>[2x]QTSVSPSKVIL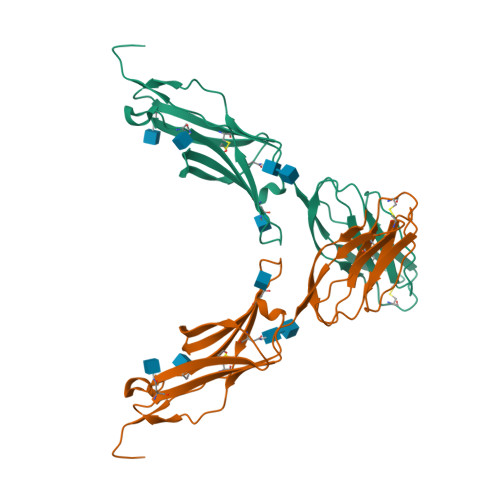PRGGSVLVTCSTSCDQPKLLGIETPLPKKELLLPGNNRKVYELSNVQEDSQPMCYSNCPDGQSTAKTFLTVYWTPERVELAPLPSWQPVGKNLTLRCQVEGGAPRANLTVVLLRGEKELKREPAVGEPAEVTTTVLVRRDHHGANFSCRTELDLRPQGLELFENTSAPYQLQTFVLPAT>GMFASLIKRFQFVSVLDSNPQTKVMSLLGTIDNKDAIITAEKTHFLFDETVRRPSQDGRSTPVLYNCENEYSCINGIQELKEITSNDIYYWGLSVIKQDMESNPTAKLNLIWPATPIHIKKYEQQNFHLVRETPEMYKRIVQPYIEEMCNNGRLKWVNNILYEGAESERVVYKDFSEENKDDGFLILPDMKWDGMNLDSLYLVAIVYRTDIKTIRDLRYSDRQWLINLNNKIRSIV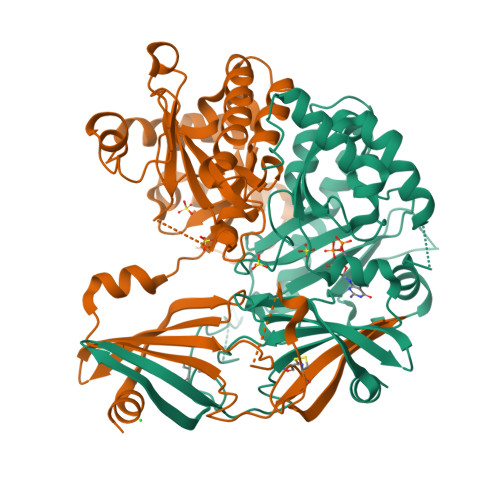PGCYNYAVHPDELRILVHYQPSYYHFNIHIVNIKHPGLGNSIAAGKAILLEDIIEMLNYLGPEGYMNKTITYAIGENHDLWKRGLEEELTKQLERDGIPKIPKIVNGFK[4x]>[4x]MDIKINDITLGNNSPFVLFGGINVLESLDSTLQTCAHYVEVTRKLGIPYIFKASFDKANRSSIHSYRGVGLEEGLKIFEKVKAEFGIPVITDVHEPHQCQPVAEVCDVIQLPAFLARQTDLVVAMAKTGNVVNIKKPQFLSPSQMKNIVEKFHEAGNGKLILCERGSSFGYDNLVVDMLG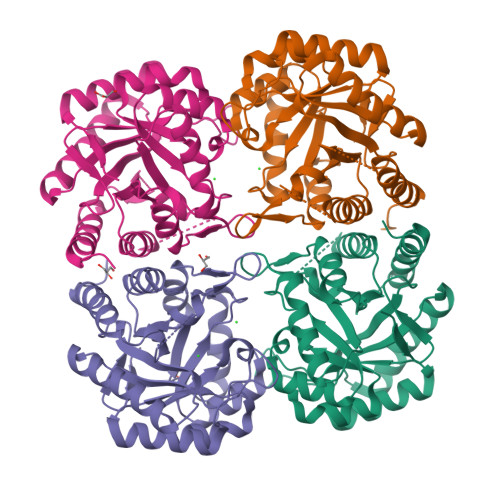FGVMKQTCGNLPVIFDVTHSLQTRDAGSAASGGRRAQALDLALAGMATRLAGLFLESHPDPKLAKCDGPSALPLHLLEDFLIRIKALDDLIKSQPILTIE>PVNTKRSNGTKRVEFPTTKKSMCIGNSTPNEQETFRAKVDEIWFRLTQKTDGTVMRDFLIEKAAEYFKQPEQPKQNAIEVISAIMAPQEEQTKSKADLYKFLAMFGPYETIMLKIASLLLISNNKGHWLTFDPQAEKNANNQRDSISGWFDQNEPNCLILKTPTGIRKIWNKPLIEATGQYLMDENGEK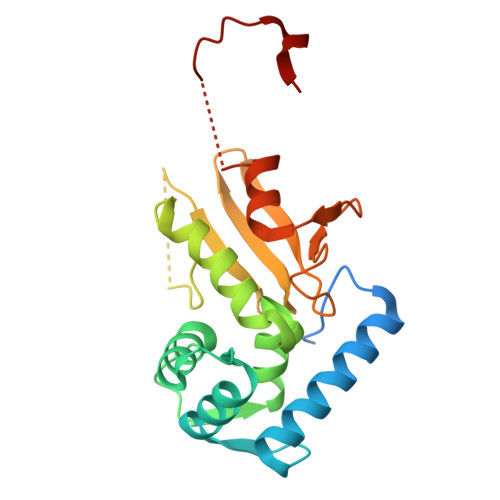YDSWDKYFEMKPIETYLTAYPTFAPMHHHHHH[2x]> MDSRLSAAYAIRAARISMIPGGVDGLVINYAEGGEPAWVQYPLKKQKPLPNNLCYTPTLE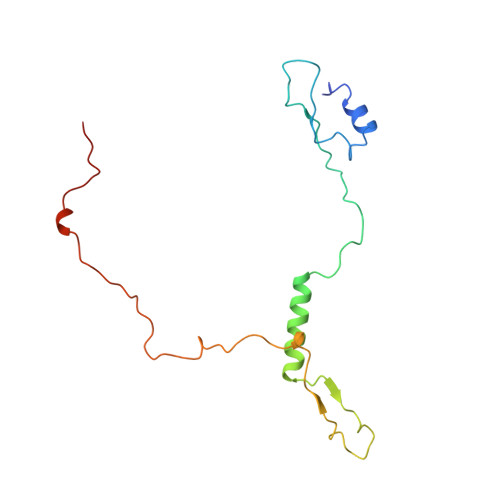DIARKREAVIAKYTKQPLETGTTFTHVLNASHLNEQYTRVKKSALPDKEFPIIETEKYPEPPILWETTIGAPSRLFDRSDGVKYVR>MQFPQLDPATLAAFSAAFRGELIWPSDADYDEARRIWNGTIDRRPALIARCTSTPDVVAAVSFARKSGLLVAVRGGGHSMAGHSVCDGGIVIDLSLMNSIKVSRRLRRARAQGGCLLGAFDTATQAHMLATPAGVVSHTGLGGLVLGGGFGWLSRKYGLSIDNLTSVEIVTADGGVLTASDTENPDLFWAVRGGGGNFGVVTAFEFDLHRVGPVRFASTYYSLDEGPQVIRAWRDHMATAPDELTWALYLRLAPPLPELPADMHGKPVICAMSCWIGDPHEGERQLESILHAGKPHGLTKATLPYRALQAYSFPGAVVPDRIYTKSGYLNELSDEATDTVLEHAADIASPFTQLELLYLGGAVARVPDDATAYPNRQSPFVTNLAAAWMDPTEDARHTAWAREGYRALAGHLSGGYVNFMNPGEADRTREA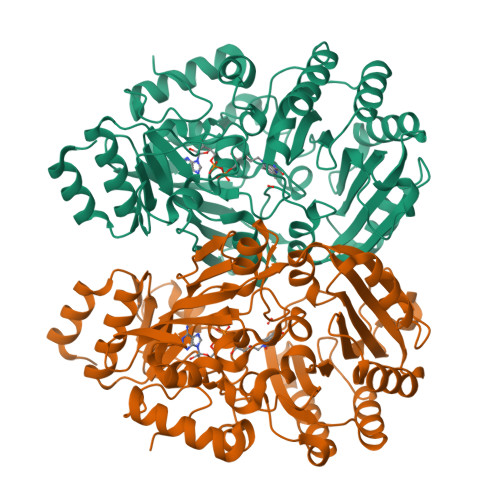YGAAKFERLQGVKAKYDPTNLFRLNQNIPPSSP[4x]Recently, we reported that the ferrous iron and 2-oxoglutarate (2OG) dependent oxygenase γ-butyrobetaine hydroxylase (BBOX) can accept substrates other than γ-butyrobetaine (GBB), and in some cases catalyzes unusual oxidative rearrangements. BBOX catalyzes the final hydroxylation step, the C3 hydroxylation of GBB, in the biosynthesis of carnitine, which is required for the transport of fatty acids into mitochondria. We report that BBOX can catalyze the oxidative desymmetrization of achiral N,N-dialkyl piperidine carboxylic acids to give products with two or three stereogenic centers. The catalytic cycle of 2OG-dependent hydroxylases involves a step in which hydrogen abstraction from the substrate is followed by hydroxylation.

The screen led to the identification of N,N-dimethyl-piperidine-4-carboxylic acid acid as a potential human BBOX substrate. NMR analysis of the reaction product resulting from the incubation of N,N-dimethyl-piperidine-4-carboxylic acid with BBOX revealed the formation of a single alcohol product: 3-hydroxy-N,N-dimethyl-piperidine-4-carboxylic acid (2). The active-site residues in the BBOX 1 NOG NiII complex are positioned similarly to those in the BBOX GBB NOG ZnII complex. At the active site, the piperidine ring of N,N-dimethyl-piperidine-4-carboxylic acid (1) is bound in a chair conformation, with its carboxylate group in the equatorial position. This result is consistent with the preferred conformation of 1 as determined by solution-phase NMR analysis. The abstracted hydrogen atom is usually observed to point towards the active-site iron center, as occurs in the complex of BBOX with NOG and GBB. In the BBOX 1 NOG NiII complex, the equatorial H3 (pro-R) atom of 1 also points towards the metal, in an orientation consistent with its abstraction in the catalytic cycle to give (3R)-hydroxy-(4S)-N,N-dimethyl-piperidine-4-carboxylic acid (2). Kinetic analysis revealed a KM value of 40 μm and a kcat value of 0.14 μm s−1 when using 1 as the BBOX substrate, compared to values of 4 μm and 0.83 μm s−1 for GBB. The results for the BBOX-catalyzed oxidation of N,N-dimethyl-piperidine-4-carboxylic acid demonstrate the potential of BBOX for the desymmetrization of cyclic achiral compounds to produce a product with two stereocenters.

> SMACTIQKAEALDGAHLMQILWYDEEESLYPAVWLRDNCPCSDCYLDSAKARKLLVEALDVNIGIKGLIFDRKKVYITWPDEHYSEFQADWLKKRCFSKQARAKLQRELFFPECQYWGSELQLPTLDFEDVLRYDEHAYKWLSTLKKVGIVRLTGASDKPGEVSKLGKRMGFLYLTFYGHTWQVQDKIDANNVAYTTGKLSFHTDYPALHHPPGVQLLHCIKQTVTGGDSEIVDGFNVCQKLKKNNPQAFQILSSTFVDFTDIGVDYCDFSVQSKHKIIELDDKGQVVRINFNNATRDTIFDVPVERVQPFYAALKEFVDLMNSKESKFTFKMNPGDVITFDNWRLLHGRRSYEAGTEISRHLEGAYADWDVVMSRLRILRQRVENGN~{N}-methyl-1,3-benzothiazole-6-carboxamide | C9 H8 N2 O S | 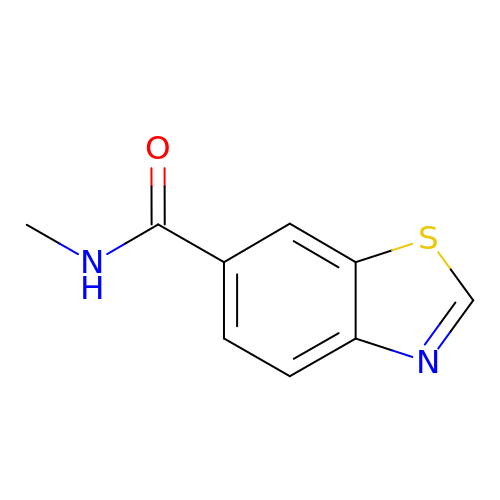KSBMLBBPMOTYRO-UHFFFAOYSA-N Poliovirus (PV), belonging to the Enterovirus genus of the Picornaviridae family, is the causative agent of poliomyelitis, an acute infectious disease that can cause paralysis, mainly in young children. PV has a positive-sense, single-stranded RNA genome encapsidated within a non-enveloped ~30 nm icosahedral protein capsid. Mature virions containing genome are composed of 60 copies each of the VP1-4 protomer; whilst in naturally occurring empty capsids (ECs) formed during PV morphogenesis VP0 remains uncleaved. The D-antigen elicits protective immune responses but can be converted to the C-antigenic form, for example by heating.

We generated PV3 SC8, containing eight stabilising mutations distributed across the VP0, VP1 and VP3 capsid proteins in the PV-IRES expression cassette in shuttle vector pMVA-PV3 SC8_PV-IRES. A total of 9,630 ‘best’ particles from 1,465 micrographs were subjected to three-dimensional (3D) reconstruction, yielding a structure to an overall resolution of 3.0 Å, as judged by a Fourier shell correlation (FSC) cut-off of 0.143. The MVA PV3 SC8 capsid was clearly in the D-antigenic conformation due to the absence of openings usually seen in the expanded state12 and the overall particle diameter of ~300 Å. The hydrophobic pocket of the VP1 capsid protein subunit was in the open state and unambiguous cryo-EM density was observed for a long-chain fatty acid molecule of ~18 carbon length bound within, which likely corresponds to the sphingosine observed bound in the native virus. This would appear to correlate with the observed stability of this variant. Disordered regions corresponding to those frequently reported for natural ECs were observed e.g. the N-terminus of VP1 from residues 1 to 65, and the N-terminus of VP0 until residue 82; including the entire region of polypeptide that would correspond to the mature VP4 protein in PV. Seven of the eight stabilising mutations were clearly distinguished in the density map, the unobserved mutation (equivalent to T67A in VP4) being located in a disordered region of VP0. The thermostability of PV3 SC8 was compared with PV3 IPV. The PV3 SC8 VLP shows significantly improved D-antigenic thermostability, maintaining 50% D-antigenicity at temperatures exceeding 60 °C. In contrast the genetically stabilised PV3 SC8 VLP was produced with high levels of D-Ag, very little C-Ag, had enhanced D-antigenic thermostability compared to IPV, and induced a neutralising antibody immune response at least as good as that from the current IPV vaccine. In contrast in the MVA expressed PV3 SC8 VLP, the pocket factor is observed at high occupancy, suggesting that the mammalian cell environment is beneficial for the synthesis of authentic particles like those produced by WPV infection of its host cells.

> MGAQVSSQKVGAHENSNRAYGGSTINYTTINYYKDSASNAASKQDYSQDPSKFTEPLKDVLIKTAPALNSPNVEACGYSDRVLQLTIGNSTITTQEAANSVVAYGRWPEFIRDDEANPVDQPTEPDVATCRFYTLDTVMWGKESKGWWWKLPDALRDMGLFGQNMYYHYLGRSGYTVHVQCNASKFHQGALGVFAIPEYCLAGDSDKQRYTSYANANPGEKGGKFYSQFNRDTAVTSPKREFCPVDYLLGCGVLLGNAFVYPHQIINLRTNNSATIVLPYVNAMAIDSMVKHNNWGIAILPLSPLDFAQESSVEIPITVTIAPMCSEFNGLRNVTAPKFQ;> GIEDLITEVAQGALTLSLPKQQDSLPDTKASGPAHSKEVPALTAVETGATNPLVPSDTVQTRHVIQRRSRSESTIESFFARGACVAIIEVDNEEPTTRAQKLFAMWRITYKDTVQLRRKLEFFTYSRFDMELTFVVTANFTNTNNGHALNQVYQIMYIPPGAPTPKSWDDYTWQTSSNPSIFYTYGAAPARISVPYVGLANAYSHFYDGFAKVPLKTDANDQIGDSLYSAMTVDDFGVLAIRVVNDHNPTKVTSKVRIYMKPKHVRVWCPRPPRAVPYYGPGVDYKDNLNPLSEKGLTTY;> GLPVLNTPGSNQYLTSDNYQSPCAIPEFDVTPPIDIPGEVKNMMELAEIDTMIPLNLENTKRNTMDMYRVTLSDSADLSQPILCFSLSPASDPRLSHTMLGEVLNYYTHWAGSLKFTFLFCGSMMATGKILVAYAPPGAQPPTSRKEAMLGTHVIWDLGLQSSCTMVVPWISNVTYRQTTQDSFTEGGYISMFYQTRIVVPLSTPKSMSMLGFVSACNDFSVRLLRDTTHISQSALPQ>MVPGACPLILRLSPTLHSADLIRDIDAMRWFLFEDTGVPLPEVNIEVLPEPTEKLTVLLYQEPVFSLSIPAQADYLLIGADASVVGDSQTLPNGMGQICWLTKDMAHKAQGFGLDVFAGSQRISALLKCVLLRHMGEFIGVQETRYLMNAMEKNYSELVKELQRQLPINKIAETLQRLVSERVSIRDLRLIFGTLIDWAPREKDVLMLTEYVRIALRRHILRRLNPEGKPLPILRIGEGIENLVRESIRQTAMGTYTALSSRHKTQILQLIEQALKQSAKLFIVTSVDTRRFLRKITEATLFDVPILSWQELGEESLIQVVESIDLSEEELADNEE[9x]

The inner membrane export gate protein, SctV (InvA in SPI-1 and SsaV in SPI-2), is the largest component of the injectisome and is essential for assembly and function of T3SS. SctV comprises a highly conserved N-terminal transmembrane (TM) domain and a less conserved C-terminal cytoplasmic domain (SctVC), which are connected via a ∼20–40 amino acid linker, SctVL, in most bacteria using the T3SS. It has been reported that SctV is one of the “engines” of T3SS; the TM domain forms a putative proton channel, and SctVC forms a nonameric ring connecting to SctN (ATPase) through SctO (the stalk protein) to function as the F0F1-ATPase, coupling energy from ATP hydrolysis and the proton-motive force to secrete unfolded bacterial effectors into the eukaryotic host. Consistent with other reported SctVC structures, the SsaVC monomer also has a four-subdomain (SD) structure and further assembles to a nonameric ring aligned to SD3, which is the most conserved region of SsaVC.

In this study, through generating a chimeric protein consisting of the TM region of InvA and the cytoplasmic region of SsaV, we produced the full-length SctV in a high-order oligomeric state which was adequate for structural study using cryo-EM single particle analysis. A homogeneous and oligomerized ISS protein was eventually obtained in buffer containing the detergent Glyco-diosgenin (GDN); however, SsaV (similarly to InvA) could not form the stable nonamer in this condition. We reconstructed a high-resolution cryo-EM structure of SsaVC with an averaged resolution of 2.11 Å. Unlike SsaVC, for which we obtained high-resolution structural information, the EM density of InvATM is blurry, and the SsaVL EM density is absent, with an approximately constant distance between the cytoplasmic domain and TM domain; this is consistent with a recent study. Structural comparison between SsaVC and InvAC in a closed conformation or its counterpart in flagellum, FlhAC, in an open conformation shows that SsaVC in a full-length context presents a semi-open conformation. The diameter of the channel at the center of the SsaVC nonamer ranges from ∼54-41 Å from the cytosolic face to the TM face. Consistent with the observation above, B-factor analysis of the SsaVC structure also shows that SD3 is the most stable region of SsaVC with the more flexible SD2 and SD4 floating around it. In each SsaVC monomer, the hydrophobic pocket at the connection region between SD1 and SD3 is occupied by a hydrophobic peptide (M346-V347-P348-G349-A350) from the neighboring SsaVL, forming the hydrophobic interactions between two adjacent subunits. Using 3D classification with this map as the reference without a local mask, the linker region was classified into variable conformations, with two major orientations, featured as left and right linkers (bottom-left panel).>MPGLFLTLEGLDGSGKTTQARRLAAFLEAQGRPVLLTREPGGGLPEVRSLLLTQELSPEAEYLLFSADRAEHVRKVILPGLAAGKVVISDRYLDSSLAYQGYGRGLPLPWLREVAREATRGLKPRLTFLLDLPPEAALRRVRRPDRLEGLGLEFFRRTREGYLALARAE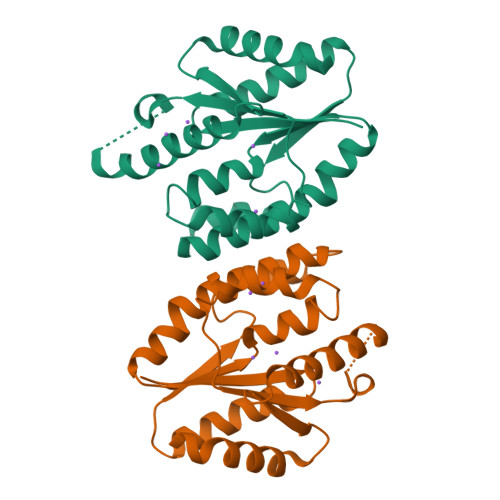PGRFVVLDATLPEEEIARAIQAHLRPLLP[2x]> GSMNTEAEQQLLHHARNGNAEEVRKLLAAMARMEVVADIDCKGRSKSNLGWTPLHLACYFGHKQVVEDLLKAGAKVNMLNDMGDTPLHRAAFTGRKELVL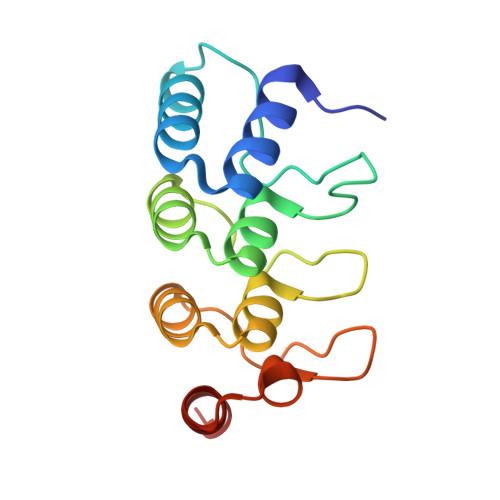LLLEYDADSTVVNGSGQTAKEATHDKEIRNMLEAVERT> GSHMTSSANEDMPVE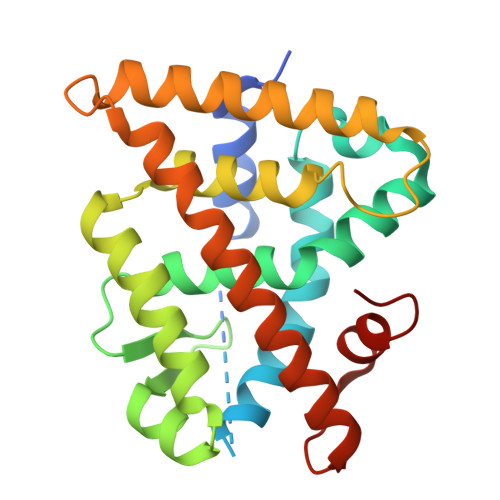RILEAELAVEPKTETYVEANMGLNPSSPNDPVTNICQAADKQLFTLVEWAKRIPHFSELPLDDQVILLRAGWNELLIASFSHRSIAVKDGILLATGLHVHRNSAHSAGVGAIFDRVLTELVSKMRDMQMDKTELGCLRAIVLFNPDSKGLSNPAEVEALREKVYASLEAYCKHKYPEQPGRFAKLLLRLPALRSIGLKCLEHLFFFKLIGDTPIDTFLMEMLEAPHQMT> NGIVPDAGHQGPDVSAVNGGTQVINIVTPNNEGISHNQYQDFNVGKPGAVLNNALEAGQSQLAGHLNANSNLNGQAASLILNEVVSRNPSFLLG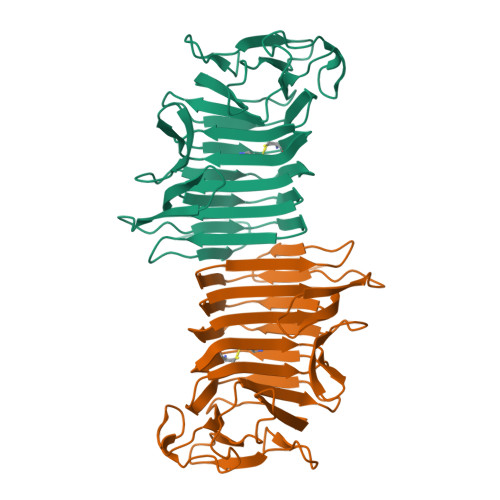QQEVFGIAAEYVLSNPNGITCDGCGFINTSRSSLVVGNPLFENGQLKGYSTLNNTNLLSLGKNGLNTTGLLDLIAPRIDSRGKITAAEISAFTGQNTFSQHFDILSSQKPVSALDSYFFGSMQSGRIRIINTAEGSGVKLAGHHHHHH> MLPKRRRARVGSPSGDAASSTPPSTRFPGVAIYLVEPRMGRSRRAFLTGLARSKGFRVLDACSSEATHVVMEETSAEEAVSWQERRMAAAPPGCTPPALLDISWLTESLGAGQPVPVECRHRLEVAGPRKGPLSPAWMPAYACQRPTPLTHHNTGLSEALEILAEAAGFEGSEGRLLTFCRAASVLKALPSPVTTLSQL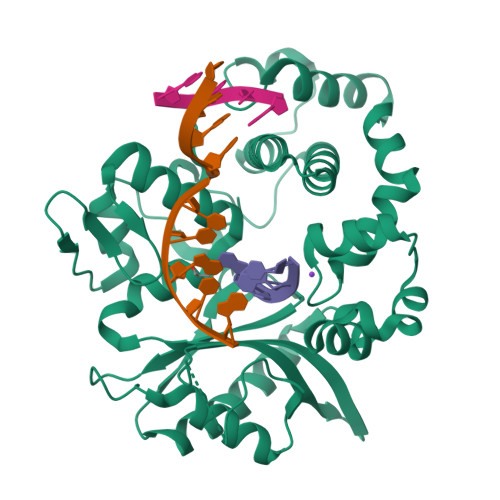QGLPHFGEHSSRVVQELLEHGVCEEVERVRRSERYQTMKLFTQIFGVGVKTADRWYREGLRTLDDLREQPQKLTQQQKAGLQHHQDLSTPVLRSDVDALQQVVEEAVGQALPGATVTLTGGFRRGKLQGHDVDFLITHPKEGQEAGLLPRVMCRLQDQGLILYHQHQHSCCESPTRLAQQSHMDAFERSFCIFRLPQPGSWKAVRVDLVVAPVSQFPFALLGWTGSKLFQRELRRFSRKEKGLWLNSHGLFDPEQKTFFQAASEEDIFRHLGLEYLPPEQRNA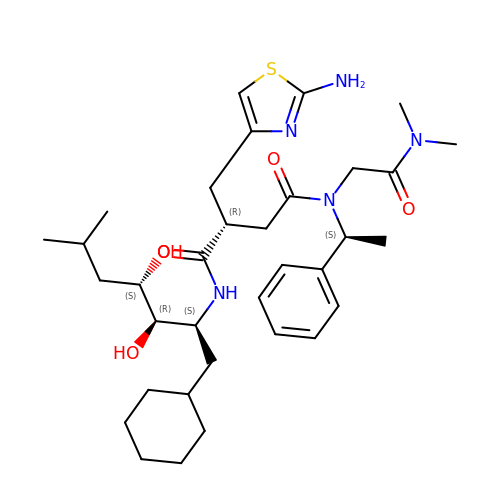(2S)-2-[(2-amino-1,3-thiazol-4-yl)methyl]-N~1~-[(1S,2R,3R)-1-(cyclohexylmethyl)-2,3-dihydroxy-5-methylhexyl]-N~4~-[2-(dimethylamino)-2-oxoethyl]-N~4~-[(1S)-1-phenylethyl]butanediamide | C34 H53 N5 O5 S | OXJHMLABLLIRCI-MKLHLGAXSA-N>MMRASFLVLAAL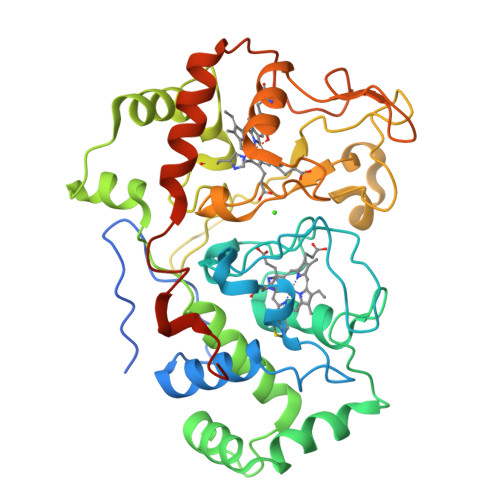VLGARSAAEPAPAWNWDLPKYIPPPRVPVDNPMSEEKFQLGRRLFYDKRLSGNGTLSCSSCHLQERAFTDGRTVSIGSTGAKTPRNAPSIAYSGWHGTLTWANPALVTLERQMLNPLFGADPIEMGASDANKAEIVARFRADADYRRWFAAAFPEMSEPISFATIIAAISAFQRGVYSFDSRYDHYLQGEAQLTEAEQRGHDLYFGEKAECHHCHGSVGLDDQFVHARTREPELPFHNTGLYDIDGKGAYPAPNHGLFDITGDPDDMGKFRAPSLRNIALTAPYMHDGSVATLEEVIDIYSEGGRKIASGPHAGDGRASALKSGLIVKIDLTAQEKADLLAFLKTLTDESLIASPRFSDPWRTPTAAKWSHPQFEK[2x]>[2x]MTETIKTDVLIVGAGPCGLFAVFELGLLDVKAHLVDILDKVGGQCAELYPEKPIYDIPGIPMVTGHGLTEALMEQIKPFNPTFHLSEMVENVEKIGDPGFRVTTNAGKVFECTVLVVAAGGGSFLPKRPPVP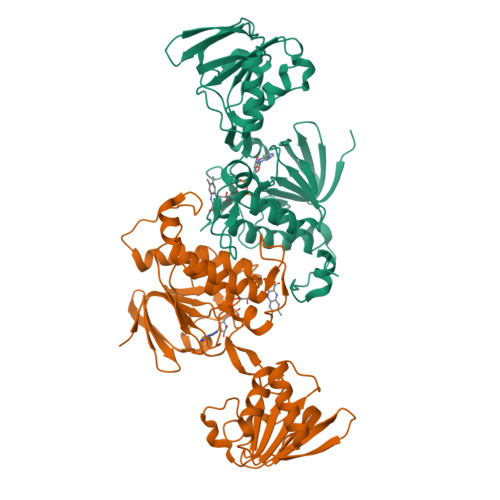GVEAYEGTSVHYAVRKMEDFRGKDILIVGGGDSALDWTLNLNPIAKSMTLVHRRDDFRGAPHSVEQMRQLVASGKLDLKIGQITELQGDNGQLTGATVKLNDNTTSQIKCDAMLPFFGLTMKLGPVANWGLDLENNLIPVDTGTFETNVPGIFAIGDINTYPGKLKLILSGFHEGALMAQKAVKYVYPDKRVVFQYTTSSTNLQKKLGVN> GGMQADKCPVTGATATTARGDSVEFDFFAAPQAYRRVAAEHRADGAFHSSRGDSFWVLSTYEGICAAFRDEDTFSVSRVSAADG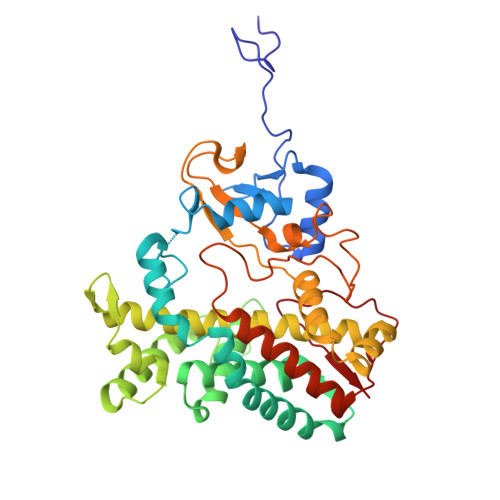AEDERWIPLTIQGRTHNEWRRRLAAWFTPQRARDLTPAIRANARRRISAFVDRGEVSFSDEFARPYVLENLMLAVGWPLADLDHLLAINVAMIRSREAPDPRQAFNAETAFPALQEYVRRHVARRRAEPVEGDLTSATFDWEIDGTPVSDADRESLLTVLFLAGVDSTVNHMANGIQHLAHHPGDRHRFLRDPEVRPAAVEEFLRVNSCMYPGRLATREGAGGVASQGDTVLLPLALANYDPAVFPEPERVDFDREQNPHIAFGTGHHQCLGAAYARAQILTAWEEWHELIPDYRLPDPTVEPPFLRNVYDLRIVW> IVGGENAKPGQFPWQVLLNGKIDAFCGGSIINEKWVVTAAHCIEPGVKITVVAGEYNTEETEPTEQRRNVIRAIPHHSYNATVNKYSHDIALLELDEPLTLNSYVTPICIADKEYTNIFLKFGSGYVSGWG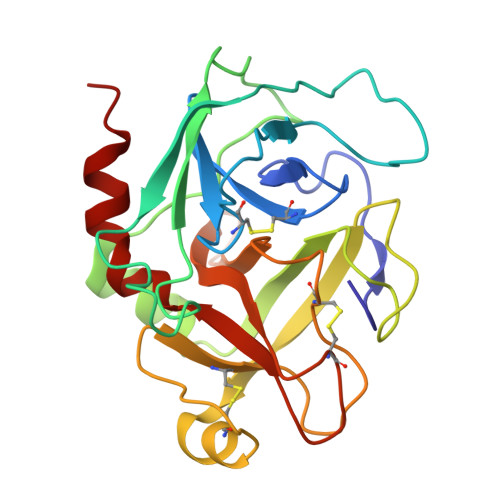RVFNRGRSATILQYLKVPLVDRATCLRSTKFTIYSNMFCAGFHEGGKDSCQGDSGGPHVTEVEGTSFLTGIISWGEECAVKGKYGIYTKVSRYVNWIKEKTKLT> TDRLKGKVAIVTGGTLGIGLAIADKFVEEGAKVVITGRHADVGEKAAKSIGGTDVIRF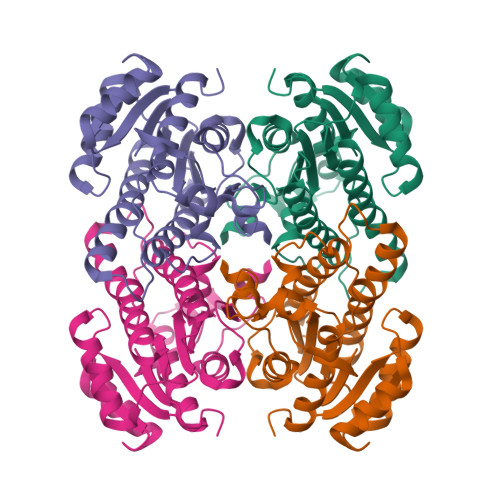VQHDASDEAGWTKLFDTTEEAFGPVTTVVNNAGIAVSKSVEDTTTEEWRKLLSVNLDGVFFGTRLGIQRMKNKGLGASIINMSSIEGFVGDPTLGAYNASKGAVRIMSKSAALDCALKDYDVRVNTVHPGYIKTPLVDDLEGAEEMMSQRTKTPMGHIGEPNDIAWICVYLASDESKFATGAEFVVDGGYTAQ N~3~-{[5-(4-acetylphenyl)-4-methyl-1,3-thiazol-2-yl]carbamoyl}-N-tert-butyl-beta-alaninamide | C20 H26 N4 O3 S | 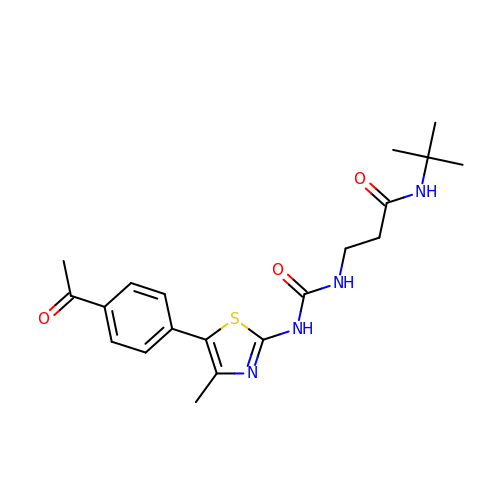IUPXLLWDLOWEBR-UHFFFAOYSA-N>[4x]ARRPSVIWLSFQECTGCTESLTRAHAPTLEDLILDFISLDYHHTLQAASGEAAEAARLQAMDENRGQYLVIVDGSIPGPDANPGFSTVAGHSNYSILMETVEHAAAVIAVGTCAAFGGLPQARPNPTGAMSVMDLVRDKPVINVPGCPPIPMVITGVIAHYLVFGRLPELDGYGRPLAFYGQSIHDRCYRRPFYDKGLFAESFDDEGAKQGWCLYRLGCKGPTTYNACATMKWNDGTSWPVEAGHPCLGCSEPQFWDAGGFYEPVSVPL;>MSERIVVDPITRIEGHLRIEAQMDGATIAQAYSSGTMVRGIETILKGRDPRDAWAFVQRICGVCTLVHGIASVRAVEDALRIELPLNAQLIRNLMIGAQYIHDHVMHFYHLHALDW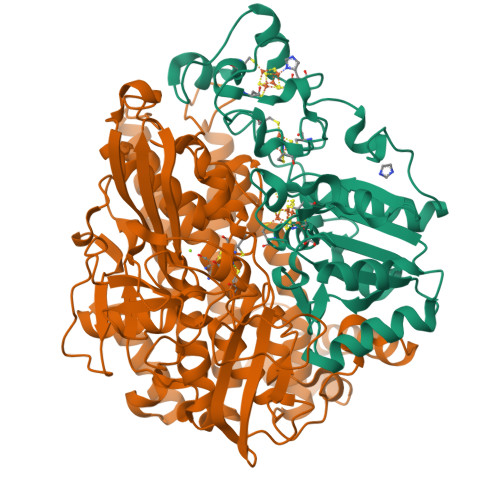VDVVSALSADPRATSELAQSISAWPKSSPGYFADTQKRIKTFVESGQLGIFANGYWGHPAYRLPPEANLMAVAHYLEALAWQRDTAKFHAIFGGKNPHPNFVVGGVPSPIDLDSDSALNAKRLAEVRNLIQSMRTFVDQVYVPDTLAIAGFYKDWGERGEGLGNFLCYGDLPTGASLDPATFLFPRGAILDRDLSTIHEVDLEATGEIQEFVNHSWYEYSVGNDRGLHPYEGQTNLEYDRRGGVAPPYKQLDVSDGYSWLKAPRWKGRSVEVGPLARVLMLYATGHDQARELVDSTLSRLDLPVDALYSTLGRTAARALESKILVDAMQGWYDGLIANVKSGDTKTFNETLWEPSSWPSRAQGVGIMEAPRGALGHWIVIEDGRIANYQAVVPSTWNAGPRDGRGQAGAYEAALQDNHQLVDVKQPIEILRTIHSFDPCIACAVH[4x]>SSTQALTYLNALQHSIRLSGVEDHVKNFRPQCLVMTGAPNSRPALLHLVHDFTKNVGLMICGHVHMGPRRQAMKEMSIDQAKYQRWLIKNKMKAFYAPVHADDLREGAQYLMQAAGLGRMKPNTLVLGFKKDWLQADMRDVDMYINLFHDAFDIQYGVVVIRLKEGLDISHLQGQESKGPIVPLNVADQKLLEASTQFQKKQGKNTIDVWWLFDDGGLTLLIPYLLTTKKKWKDCKIRVFIGGKINRIDHDRRAMATLLSKFRIDFSDIMVLGDINTKPKKENIIAFEEIIEPYRLHEDDKEQDIADKMKEDEPWRITDNEL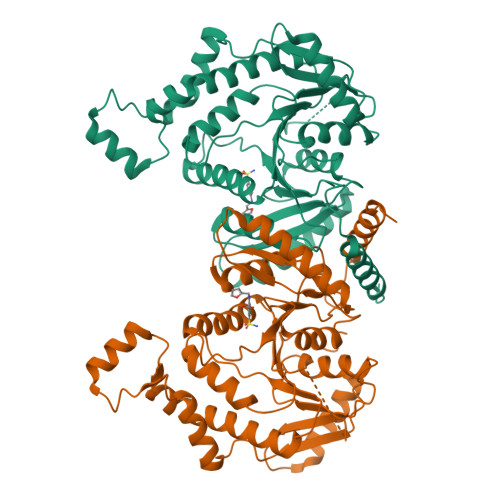ELYKTKTYRQIRLNELLKEHSSTANIIVMSLPVARKGAVSSALYMAWLEALSKDLPPILLVRGNHQSVLTF[2x]> MTIEELKTRLHT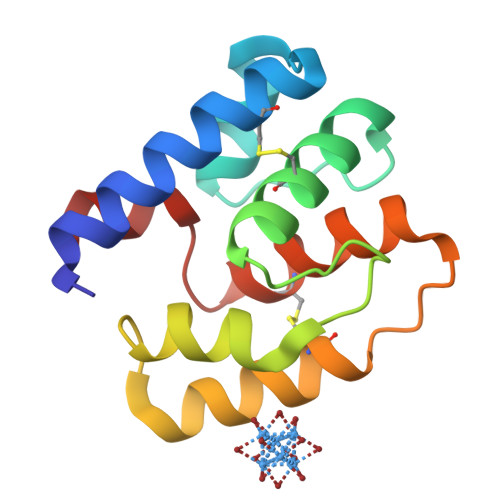EQSVCKTETGIDQQKANDVIEGNIDVEDKKVQLYCECILKNFNILDKNNVFKPQGIKAVMELLIDENSVKQLVSDCSTISEENPHLKASKLVQCVSKYKTMKSVDFL The TLP Gentlyase, the neutral metalloprotease from Paenibacillus polymyxa (EC 3.4.24.28), is an extracellular metalloprotease that cleaves fibronectin, collagen IV and, to a lesser extent, collagen and has maximum activity at neutral pH. This enzyme is used to gently disperse mammalian cells and tissues and is widely applied in cell-culture procedures or for the isolation and tissue dissociation of primary cells. The Gentlyase metalloprotease structure shows the overall architecture of a typical TLP. The C-terminal and N-terminal domains are connected by a central α-helix containing several catalytically crucial residues.

Here, we report (i) a method that can be generally applied to identify suitable conditions to keep active TLP stable for crystallization and (ii) the structure of Gentlyase, the TLP of P. polymyxa, at 1.59 Å resolution in the absence of and at 1.76 Å resolution in the presence of phosphoramidon, the natural TLP inhibitor from Streptomyces tanashiensis. The only significant difference from the thermolysin phosphoramidon binding is observed in the rhamnose group of the inhibitor. The same phosphoramidon conformation is also observed in both independent copies in the Gentlyase crystal. However, the observed rhamnose conformation is also influenced by crystallization, because the rhamnose groups of both phosphoramidons in the crystallo­graphic asymmetric unit are involved in different crystal lattice contacts. In one instance the phosphoramidon hydroxy group O4 hydrogen bonds to Tyr151 and in the second instance hydroxy group O3 hydrogen bonds to Asn221 of a different crystal lattice neighbour. Because no domain movement was observed upon inhibitor binding, as for thermolysin and for aureolysin, the domain movement upon inhibitor binding observed in B. cereus TLP could not be confirmed as a general feature of TLPs. To prevent autolysis, the phosphoramidon-inhibited protease complex was first prepared in both a calcium-depleted and a calcium-containing form and both were then analyzed in a thermal unfolding assay. The calcium-depleted inhibited metalloprotease showed a significantly reduced apparent melting temperature of 337 K compared with 347 K for the calcium-containing enzyme in 100 mM CaCl2. Comparison with other TLPs showed that the marked calcium dependency of Gentlyase stability may arise from a partly degenerated calcium site Ca1–2 and a deletion near site Ca3.

>ATGTGKGVLGDTKSFTTTASGSSYQLKDTTRGNGVVTYTASNRQSIPGTILTDADNVWNDPAGVDAHTYAAKTYDYYKAKFGRNSIDGRGLQLRSTVHYGSRYNNAFWNGSQMTYGDGDGSTFIAFSGDPDVVGHELTHGVTEYTSNLEYYGESGALNEAFSDVIGNDIQRKNWLVGDDIYTPNIAGDALRSMSNPTLYDQPDHYSNLYTGSSDNGGVHTNSGIINKAYYLLAQGGTFHGVTVNGIGRDAAVQIYYSAFTNYLTSSSDFSNARAAVIQAAKDQYGANSAEATAAAKSFDAVGVN[2x]>GSRPTDIKCSASYQCFPVCKSRFGKTNGRCVNGLCDCF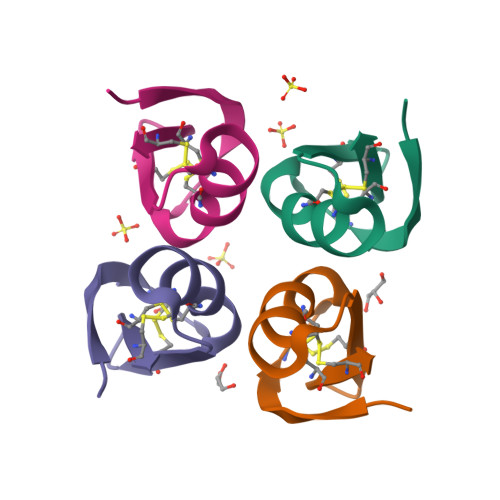[4x]>YMIQEEEWDRDLLLDPAWEKQQRKTFTAWCNSHLRKAGTQIENIEEDFRNGLKLMLLLEVISGERLPKPDRGKMRFHKIANVNKALDYIASKGVKLVSIGTEEIVDGNVKMTLGMIWTIILRFAIQDISVEETSAKEGLLLWCQRKTAPYRNVNIQNFHTSWKDGLGLCALIHRHRPDLIDYSKLNKDDPIGNINLAMEIAEKHLDIPKMLDAEDIVNTPKPDERAIMTYVSCFYHA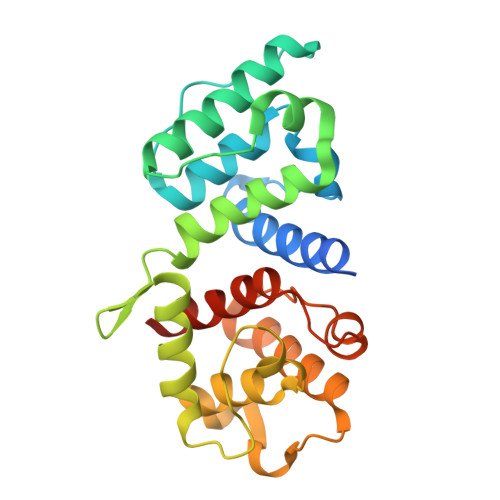FAGAEQAETAA[2x]>MRNEMHLQFSARSENESFARVTVAAFVAQLDPTMDELTEIKTVVSEAVTNAIIHGYNNDPNGIVSISVIIEDGVVHLTVRDEGVGIPDIEEARQPLFTTKPELERSGMGFTIMENFMDEVIVESEVNKGTTVYLKKHIVKSKALSN[3x];>[3x]GSHMSLAIDLEVKQ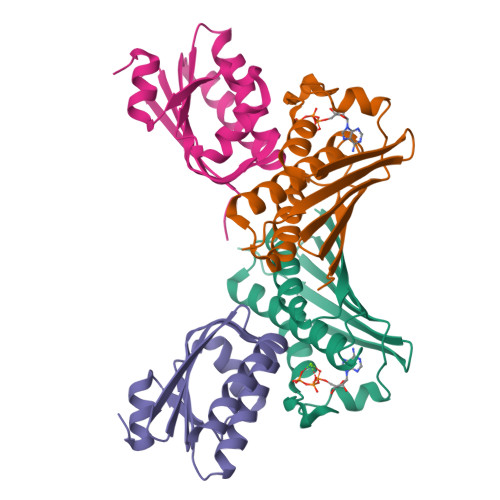DVLIVRLSGELDHHTAEELREQVTDVLENRAIRHIVLNLGQLTFMDASGLGVILGRYKQIKNVGGQMVVCAVSPAVKRLFDMSGLFKIIRVEADEQFALQALGVA> MIQLFDYYNQETQDLHDSLLAAGYACPTIVIEANGFLPDDMISPYTYFLGDEEGVDHPLFFNQVPVPPFWEITGDHQVARVSDMGEERARIHYASQARGRLVKQVDWLDKKGQ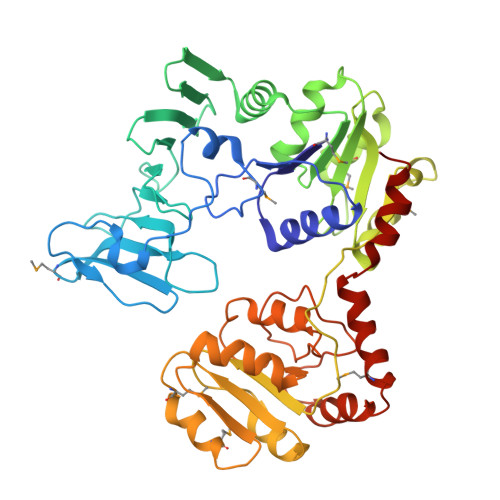LRLSERYNKQGRCFAKTAYKSGQEAFNTTYYSTDGQERIVENHVTGDIILTLDQEPLRIFKSRVDFIRFFLERLDLDLDHILFNSLAYSFLVSHSLTGRAGQDILFWQEPLYDELPGNMQLILDNSQLRTQTIVIPDLATYEKAMSLAAADQQQKFLHLGYHYDFKRDNYLRKDALILTHSDQIEGLDTLVQSLPQLVFRIAALTEMSPKLLSMLSYKNVVLYQNASLKQIEQLYLESDIYLDINHGGQVLQAVRKAFENNLLILGFEQTLHDRHYIAQQHIFDSSQPAQLASILEEALCGVEQMRSALQAQGRHANDVPVSLYQETLQSLLG> EGVAAALTPERLLEWQDKGIFVIQSESLKKCIQAGKSVLTLENCKQANKHMLWKWVSNHGLFNIGGSGCLGLNFSAPEQPLSLYECDSTLVSLRWRCNRKMITGPLQYSVQVAHDNTVVASRKYIHKWISYGSGGGDICEYLHKDLHTIKGNTHGMPCMFPFQYNHQWHHECTREGREDDLLWCATTSRYERDEKWGFCPDPTSAEVGCDTIWEKDLNSHICYQFNLLSSLSWSEAHSSCQMQGGTLLSITDETEENFIREHMSSKTVEVWMGLNQLDEHAGWQWSDGTPLNYLNWSPEVNFEPFVEDHCGTFSSFMPSAWRSRDCESTLPYICKKYLNHIDHEIVEKDAWKYYATHCEPGWNPYNRNCYKLQKEEKTWHEALRSCQADNSALIDITSLAEVEFLVTLLGDENASETWIGLSSNKIPVSFEWSNDSSVIFTNWHTLEPHIFPNRSQLCVSAEQSEGHWKVKNCEERLFYICKKAGHVLSDAESGCQEGWERHGGFCYKIDTVLRSFDQASSGYYCPPALVTITNRFEQAFITSLISSVVKMKDSYFWIALQDQNDTGEYTWKPVGQKPEPVQYTHWNTHQPRYSGGCVAMRGRHPLGRWEVKHCRHFKAMSLCKQPVENQEKAEYEERWPFHPCYLDWESEPGLASCFKVFHSEKVLMKRTWREAEAFCEEFGAHLASFAHIEEENFVNELLHSKFNWTEERQFWIGFNKRNPLNAGSWEWSDRTPVVSSFLDNTYFGEDARNCAVYKANKTLLPLHCGSKREWICKIPRDVKPKIPFWYQYDVPWLFYQDAEYLFHTFASEWLNFEFVCSWLHSDLLTIHSAHEQEFIHSKIKALSKYGASWWIGLQEERANDEFRWRDGTPVIYQNWDTGRERTVNNQSQRCGFISSITGLWGSEECSVSMPSICKRKKVWLIEKKKDTPKQHGTCPKGWLYFNYKCLLLNIPKDPSSWKNWTHAQHFCAEEGGTLVAIESEVEQAFITMNLFGQTTSVWIGLQNDDYETWLNGKPVVYSNWSPFDIINIPSHNTTEVQKHIPLCALLSSNPNFHFTGKWYFEDCGKEGYGFVCEKMQDTSGHGVNTSDMYPMPNTLEYGNRTYKIINANMTWYAAIKTCLMHKAQLVSITDQYHQSFLTVVLNRLGYAHWIGLFTTDNGLNFDWSDGTKSSFTFWKDEESSLLGDCVFADSNGRWHSTACESFLQGAICHVPPETRQSEHPELCSETSIPWIKFKSNCYSFSTVLDSMSFEAAHEFCKKEGSNLLTIKDEAENAFLLEELFAFGSSVQMVWLNAQFDGNNETIKWFDGTPTDQSNWGIRKPDTDYFKPHHCVALRIPEGLWQLSPCQEKKGFICKMEADIHTAEALPEK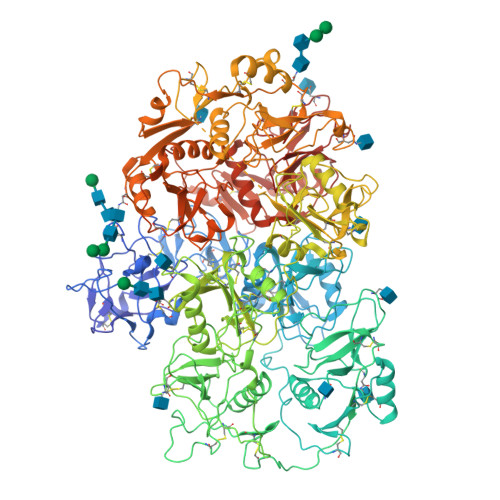GPSHS> SPREQDRFLPIANVSRIMKKALPANAKISKDAKETMQECVSEFISFVTGEASDKCQKEKRKTINGDDLLWA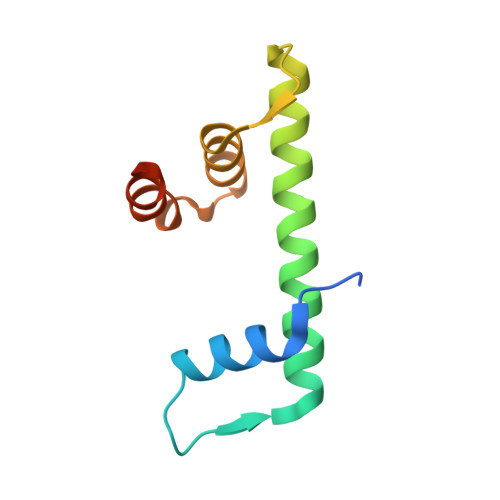MTTLGFEDYVEPLKVYLQRFREIEGE> MSFFHGVTVTNVDIGARTIALPASSVIGLCDVFTPGAQASAKPNVPVLLTSKKDAAAAFGIGSSIYLACEAIYNRAQAVIVAVGVETAETPEAQASAVIGGISAAGERTGLQALLDGKSRFNAQPRLLVAPGHSAQQAVATAMDGLAEKLRAIAILDGPNSTDEAAVAYAKNFGSKRLFMVDPGVQVWDSATNAARNAPASAYAAGLFAWTDAEYGFWSSPSNKEIKGVTGTSRPVEFLDGDETCRANLLNNANIATIIRDDGYRLWGNRTLSSDSKW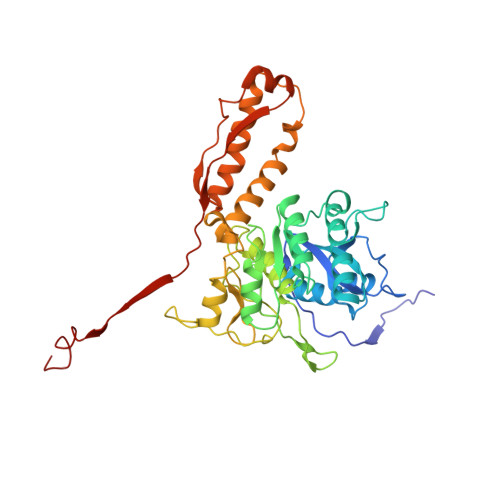AFVTRVRTMDLVMDAILAGHKWAVDRGITKTYVKDVTEGLRAFMRDLKNQGAVINFEVYADPDLNSASQLAQGKVYWNIRFTDVPPAENPNFRVEVTDQWLTEVLDVA>PPGPPGPPGPPG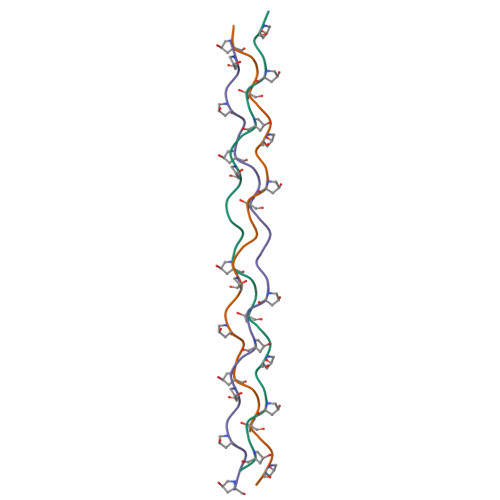EKGPPGPPGPPGPPGPPG[3x]> MCDLRKTKLIDKISSLELYKYSIFFRNYIENVAEDCLKNGLILE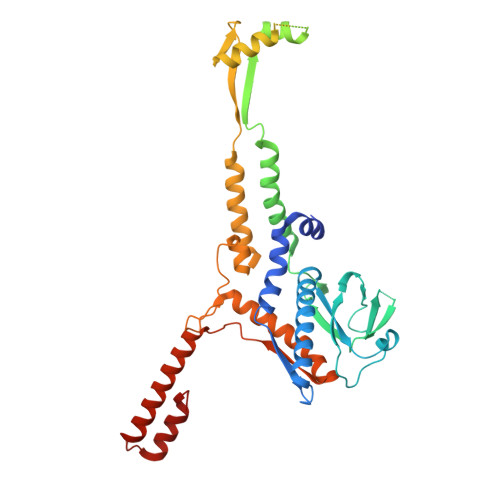SAAHNVSEVELARLKVQLKNALLNCIISYRFHGIGYVLVKTKDTLIDLEQPVNIELPIGFEYLDYEYVRDLGVDFDHITYKVKSNNKNNSLDAVKIHKSRLIIYENFDYILKRYVPCYTESFLLDIYLFEKIYVEIERRIENHNFLFYKDESLVQLQDALSSATTSLSALTQSNNDRGSGILSSFLRKQNSNNHSKDISNLRNLNDSLSQELARLKSNLNNEGMFYTATPSASLEVIKYDLSYLKEALALIKAKIGADTKEPLTRSFNEQAKGLGNDGKGDRSNYYDFLKGVQEQVENSCNLKLTKYFGLDMKFNSLIMLSEEQKVERDIKLIELYSKYNQLIQSSSFNNEELAMLKEKLFSF>MAGLPDQRLANEALKRGDTVTAQQNYQQLAELGYSEAQVGLADIQVGTRDPAQIKQAEATYRAAADTSPRAQARLGRLLAAKPGATEAEHHEAESLLKKAFANGEGNTLIPLAMLYLQYPHSFPNVNAQQQISQWQAAGYPEAGLAQVLLYRTQGTYDQHLDDVERICKAALNTTDICYVELATVYQKKQQPEQQAELLKQMEAGVSRGTVTA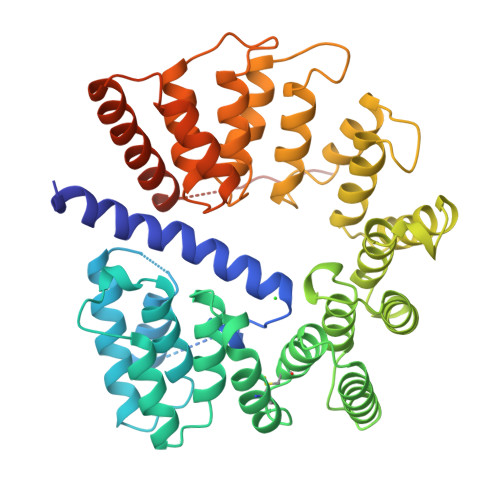QRVDSVARVLGDATLGTPDEKTAQALLEKIAPGYPASWVSLAQLLYDFPELGDVEQMMKYLDNGRAADQPRAELLLGKLYYEGKWVPADAKAAEAHFEKAVGREVAADYYLGQIYRRGYLGKVYPQKALDHLLTAARNGQNSADFAIAQLFSQGKGTKPDPLNAYVFSQLAKAQDTPEANDLATQLEAPLTPAQRAEGQRLVQQELAARGTLAQSTLQLHALQEEDGEESLLEHHHHHH[4x]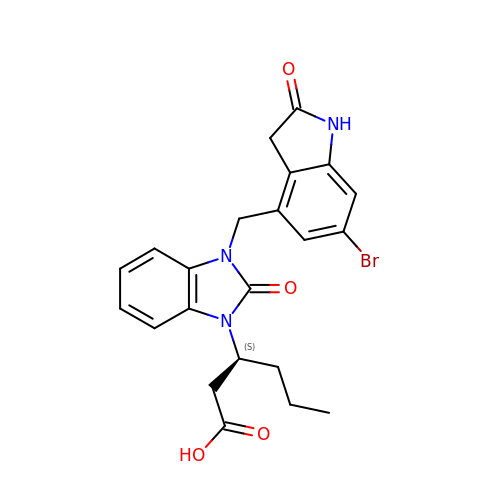(3S)-3-{3-[(6-bromo-2-oxo-2,3-dihydro-1H-indol-4-yl)methyl]-2-oxo-2,3-dihydro-1H-benzimidazol-1-yl}hexanoic acid | C22 H22 Br N3 O4 | HGSJUJNYFCUFGB-HNNXBMFYSA-N>[6x]GPMFEARLVQGSILKKVLEALKDLINEACWDISSSGVNLQSMDSSHVSLVQLTLRSEGFDTYRCDRNLAMGVNLTSMSKILKCAGNEDIITLRAEDNADTLALVFEAPNQEKVSDYEMKLMDLDVEQLGIPEQEYSCVVKMPSGEFARICRDLSHIGDAVVISCAKDGVKFSASGELGNGNIKLSQTSNVDKEEEAVTIEMNEPVQLTFALRYLNFFTKATPLSSTVTLSMSADVPLVVEYKIADMGHLKYYLAPKIEDEEGS;>MEQRRVTDFFARRR[6x]

The CRL4Cdt2 ubiquitin ligase complex is an essential regulator of cell-cycle progression and genome stability, ubiquitinating substrates such as p21, Set8, and Cdt1, via a display of substrate degrons on proliferating cell nuclear antigens (PCNAs). In contrast, CRL4Cdt2 recognizes Cdt1 when bound to the proliferating cell nuclear antigen (PCNA) trimer, through a binding motif (PIP box) in its N-terminal end. Unexpectedly, we found a PIP box in the C-terminal end of Cdt2, and showed that it directly mediates interaction of Cdt2 with PCNA. X-ray crystallographic structures of PCNA bound to Cdt2PIP and Cdt1PIP show that the peptides occupy all three binding sites of the trimeric PCNA ring.

As Cdt1 is recruited to PCNA on chromatin during the S phase and after DNA damage through the Cdt1 N-terminal PIP box (residues 3–10), we then synthesized a Cdt1PIP-TAMRA (MEQRRVTDFFARRR) peptide, to compare its affinity with PCNA. Remarkably, the affinity of the Cdt1PIP peptide to PCNA (7, 200 ± 200 nM) is two orders of magnitude weaker than that for the Cdt2PIP, and similar to what is reported for other peptides derived, for example, from the pol-δ p66 and FEN1 (1–60 μM). To confirm the binding mode of the Cdt2PIP and Cdt1PIP peptides to PCNA, we determined the crystal structure of both complexes by X-ray crystallography, to a 3.5- and 3.4-Å resolution, respectively. PCNA adopts its well-characterized trimer conformation, with one peptide bound per monomer. The binding mode of both the peptides was very clear (see the Materials and Methods section for details). Both peptides bind in a similar manner to other PCNA complex structures. Some notable differences in the binding mode are the conserved Phe713/Phe11 side-chain ring that rotates 180 degrees between the two structures and the Tyr712/Phe10 that repositions so as to extend more towards a hydrophilic environment in Cdt2. The Ile709 and Val7 side chains occupy a similar space in the hydrophobic recognition pocket. Albeit the peptide main chain is in a very similar conformation between the structures, some of the other side chains adopt rather different conformations. The average buried area upon the binding of the Cdt2 peptide is 692 ± 6 Å2 and average calculated energy of binding is −13 ± 0.2 kcal·mol−1, whereas the average buried area upon the binding of the Cdt1 peptide is 650 ± 4 Å2 and average calculated energy of binding is −8.3 ± 0.5 kcal·mol−1; these confirm the tighter binding of the Cdt2 peptide to PCNA. In addition, weaker affinity of Cdt1 PIP box can help to release Cdt1 after poly-ubiquitination, whereas CRL4Cdt2 could remain on PCNA to trap the next substrate, leading to an efficient degradation cycle of substrates.>SNAMTNWLIAYQGEPGAYSEIAALRFGEPLPCESFDDVFSAVTEQKADYAVIPIENSLGGSIHQNYDLLLRRPVVILAETFVKVEHCLLGLPGASVETATKAMSHPQALVQCHN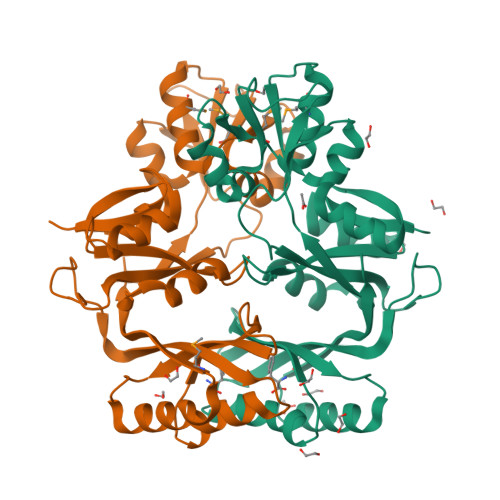FFATHPQIRAEAAYDTAGSAKMVAESRDKSALAIASKRAGELYGLDILKENLADEEWNITRFFCIAHENNPDISHLKVRPDVARQKTSIVFALPNEQGSLFRALATFALRGIDLTKIESRPSRKKAFEYLFYADFIGHREDQNVHNALENLREFATMVKVLGSYGVVNP[2x]>GPLGSMMMARKQDVRIPTYNISVVGLSGTEKEKGQCGIGKSCLCNRFVR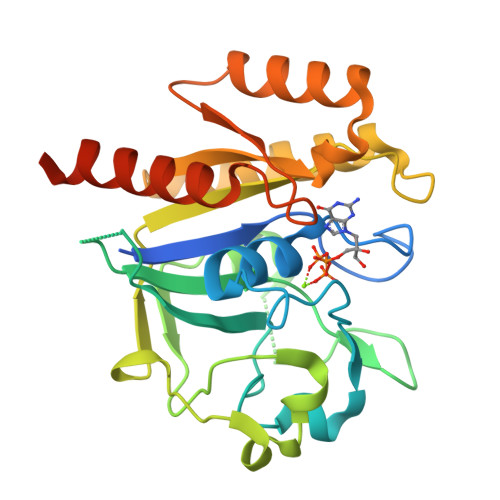PSADEFHLDHTSVLSTSDFGGRVVNNDHFLYWGEVSRSLEDCVECKMHIVEQTEFIDDQTFQPHRSTALQPYIKRAAATKLASAEKLMYFCTDQLGLEQDFEQKQMPDGKLLVDGFLLGIDVSRGMNRNFDDQLKFVSNLYNQLAKTKKPIVIVLTKCDEGVERYIRDAHTFALSKKNLQVVETSARSNVNVDLAFSTLVQLIDKSRGKTKIIPYFEALKQQ[2x]> TMGGDALRVPFLDFATATPKRHQTVVPGVGTLHDCCEHSPLFSAVARRLLFNSLVPAQLKGRDFGGDHTAKLEFLAPELVRAVARLRFKECAPADVVPQRNAYYSVLNTFQALHRSEAFRQLVHFVRDFAQLLKTSFRASSLTETTGPPKKRAKVDVATHGRTYGTLELFQKMILMHATYFLAAVLLGDHAEQVNTFLRLVFEIPLFSDAAVRHFRQRATVFLVPRRHGKTWFLVPLIALSLASFRGIKIGYTAHIRKATEPVFEEIDACLRGWFGSARVDHVKGETISFSFPDGSRSTIVFASSHNTNGIRGQDFNLLFVDEANFIRPDAVQTIMGFLNQANCKIIFVSSTNTGKASTSFLYNLRGAADELLNVVTYICDDHMPRVVTHTNATACSCYILNKPVFITMDGAVRRTADLFLADSFMQEIIG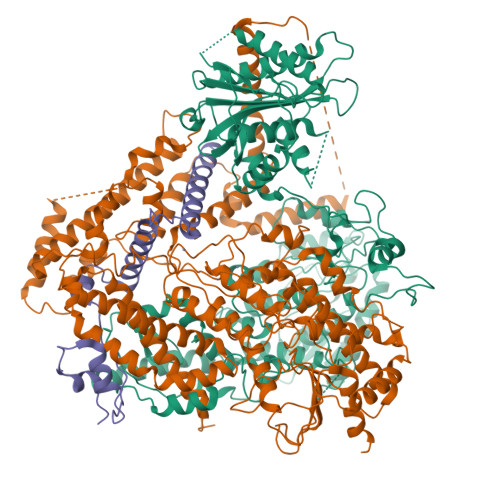GQARETGDDRPVLTKSAGERFLLYRPSTTTNSGLMAPDLYVYVDPAFTANTRASGTGVAVVGRYRDDYIIFALEHFFLRALTGSAPADIARCVVHSLTQVLALHPGAFRGVRVAVEGNSSQDSAVAIATHVHTEMHRLLASEGADAGSGPELLFYHCEPPGSAVLYPFFLLNKQKTPAFEHFIKKFNSGGVMASQEIVSATVRLQTDPVEYLLEQLNNLTETVSPNTDVRTYSGKRNGASDDLMVAVIMAIYLAAQAGPPHTF;> AAPVSEPTVARQKLLALLGQVQTYVFQIELLRRCDPHIGRGKLPQLKLNALQVRALRRRLRPGLEAQAGAFLTPLSVTLELLLEYAWREGERLLGSLETFATAGDVAAFFTETMGLARPCPYHQRVRLDTYGGTVHMELCFLHDVENFLKQLNYCHLITPSRGATAALERVREFMVGAVGSGLIVPPELSDPSHPCAVCFEELCVTANQGATIASRLADRICNHVTQQAQVRLDANELRRYLPHAAGLSDADRARALSVLDHALARTAGGDGQPHPSPENDSVRKEADALLEAHDVFQATTPGLYAISELQFWLASGDRAGQTTMDAFASNLTALARRELQQETAAVAVELALFGRRAEHFDRAFGSHLAALDMVDALIIGGQATSPDDQIEALIRACYDHHLTTPLLRRLVSPEQCDEEALRRVLARMGAGGAADAPKGGAGPDDDGDRVAVEEGARGLGAPGGGGEDEDRRRGPGGQGPETWGDIATQAAADVRERRRLYADRLTKRSLASLGRCVREQRGELEKMLRVSVHGEVLPATFAAVANGFAARARFCALTAGAGTVIDNRSAPGVFDAHRFMRASLLRHQVDPALLPSITHRFFELVNGPLFDHSTHSFAQPPNTALYYSVENVGLLPHLKEELARFIMGAGGSGADWAVSEFQRFYCFDGISGITPTQRAAWRYIRELIIATTLFASVYRCGELELRRPDCSRPTSEGRYRYPPGVYLTYDSDCPLVAIVESAPDGCIGPRSVVVYDRDVFSILYSVLQHLAPR;> TLRDTIPDCALRSQTLESLDARYVSRDGAHDAAVWFEDMTPAELEVVFPTTDAKLNYLSRTQRLASLLTYAGPIKAPDDAAAPQTPDTACVHGELLARKRERFAAVINRFLDLHQILR>MRGSPHHHHHHGSAKNVVLDHDGNLDDFVAMVLLASNTEKVRLIGALCTDADCFVENGFNVTGKIMCLMHNNMNLPLFPIGKSAATAVNPFPKEWRCLAKNMDDMPILNIPENVELWDKIKAENEKYEGQQLLADLVMNSEEKVTICVTGPLSNVAWCIDKYGEKFTSKVEECVIMGGAVDVRGNVFLPSTDG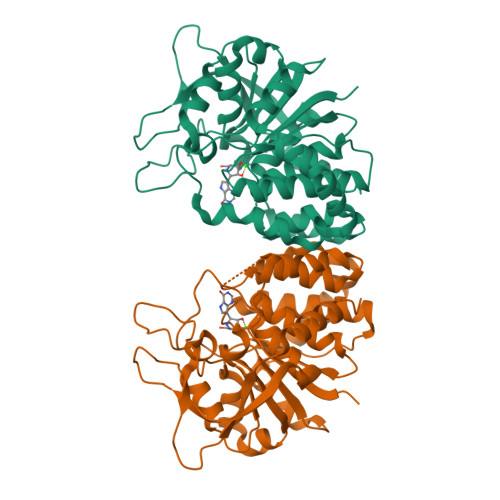TAEWNIYWDPASAKTVFGCPGLRRIMFSLDSTNTVPVRSPYVQRFGEQTNFLLSILVGTMWAMCTHCELLRDGDGYYAWDALTAAYVVDQKVANVDPVPIDVVVDKQPNEGATVRTDAENYPLTFVARNPEAEFFLDMLLRSARAC[2x]>[4x]MARKYFVAANWKCNGTLESIKSLTNSF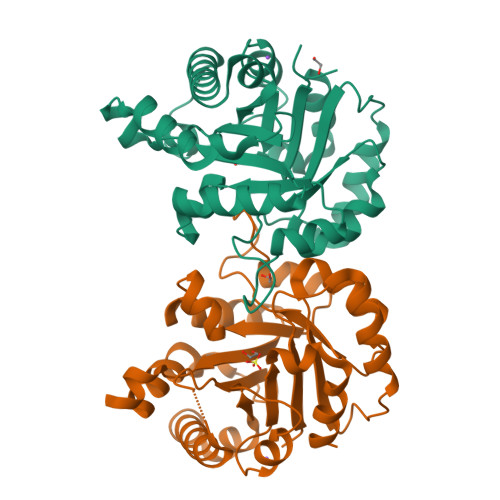NNLDFDPSKLDVVVFPVSVHYDHTRKLLQSKFSTGIQNVSKFGNGSYNGEVSAEIAKDLNIEYVIIGHFERRKYFHETDEDVREKLQASLKNNLKAVVCFGESLEQREQNKTIEVITKQVKAFVDLIDNFDNVILVYEPLWAIGTGKTATPEQAQLVHKEIRKIVKDTCGEKQANQIRILYGGSVNTENCSSLIQQEDIDGFLVGNASLKESFVDIIKSAM3-(4'-hydroxybiphenyl-4-yl)-2,4-dihydroindeno[1,2-c]pyrazol-6-ol 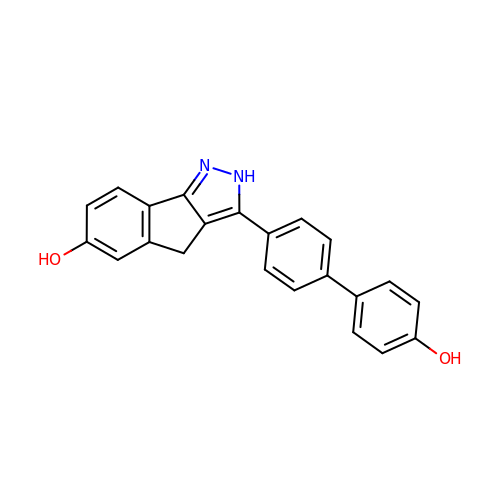| C22 H16 N2 O2 | YHNRFNJYCLUDHD-UHFFFAOYSA-N> SILYAGPTFTHSPAASNL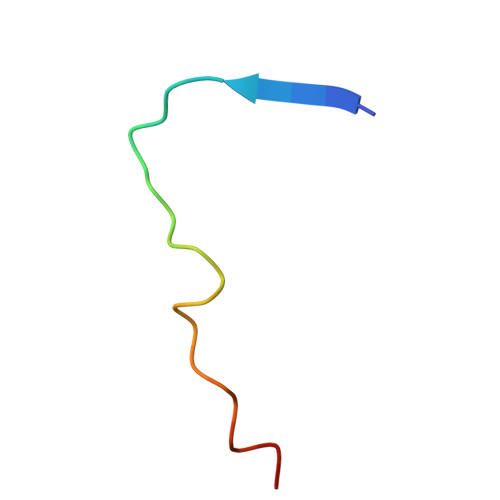PIPTFLHS>NSRVSDLDLELLFQDRAARLGKSISRLIVVASLIDKPTNLGGLCRTCEV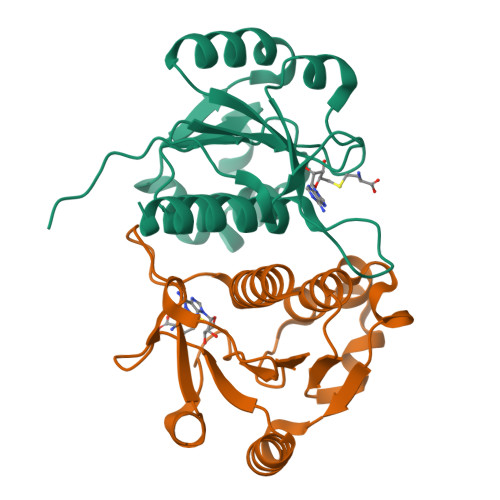FGASVLVVGSLQCISDKQFQHLSVSAEQWLPLVEVKPPQLIDYLQQKKTEGYTIIGVEQTAKSLDLTQYCFPEKSLLLLGNEREGIPANLIQQLDVCVEIPQQGIIRSLNVHVSGALLIWEYTRQQLLSHGDTKP[2x]> MESKKRQWALEDFEIGRPLGKGKFGNVYLAREKQSKFILALKVLFKAQLEKAGVEHQLRREVEIQSHLRHPNILRLYGYFHDATRVYLILEYAPLGTVYRELQKLSKFDEQRTATYITELANALSYCHSKRVIHRDIKPENLLLGSAGELKIADFGWSVHAPSSRRTTLAGTLDYLPPEMIEGRMHDEKVDLWSLGVLCYEFLVGKPPFEANTYQETYKRISRVEFTFPDFVTEGARDLISRLLKHNPSQRPMLREVLEHPWITANSSKPSNAQNKESASKQS;> SSYSYDAPSDFINFSSLDDEGDT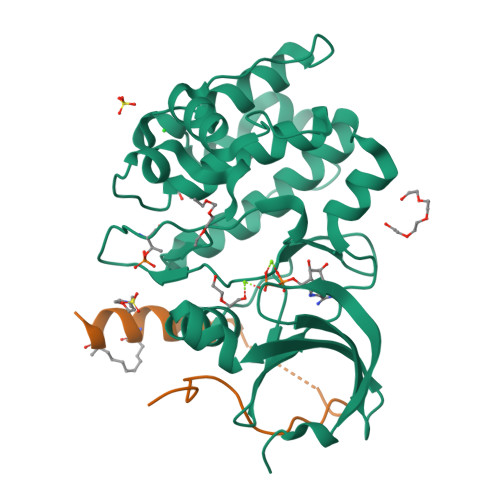QNIDSWFELKANLENX> MGEQPIFTTRAHVFQIDPSTKKNWVPASKQAVTVSYFYDVTRNSYRIISVDGAKVIINSTITPNMTFTKTSQKFGQWADSRANTVFGLGFSSELQLTKFAEKFQEVR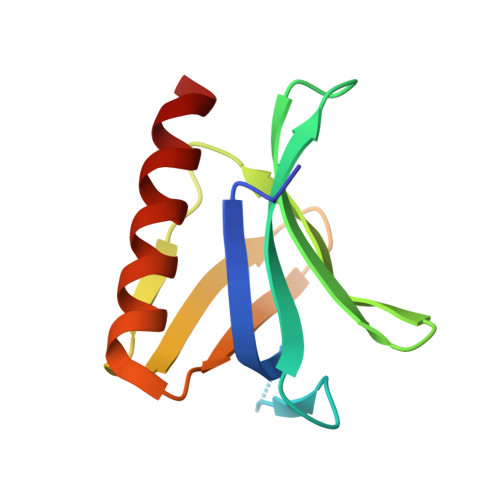EAAR>MSEDLRVGLFPVRYLVGTGLPGAPQLVLDLMVDTVDHSVVGRAAVSQAVSPPLNFHADVWGSYVFRLGPPPRRDGSGAIVQISLQGNQGGPQSNSMITFYGELLLKGDGKTGVASYRYYSNGSWHEVENVPVKADPELVPIEPGPVIGQSSMSAIGSAAMYGVAIQSAAASGDLAHMRTLSAYARQQLESRDEIAAALSELKAEIAKLESRQHHHHHH[2x]

The Q63NT7 protein from Burkholderia pseudomallei is 212 amino acids in length (molecular mass 22.5 kDa). It contains two predicted domains: an N-terminal domain of unknown function (14.5 kDa; DUF1842) and the C-terminal domain (DUF1843; 5.4 kDa), which tends to appear in multiple paralogous copies within individual bacterial operons. The N-terminal domain was predicted to fold into a β-barrel composed of eight antiparallel strands. Polar residues are found covering the exterior surface of the β-barrel, while the interior of the β-barrel is lined with mostly hydrophobic residues, without space for a channel through the barrel.

Finally, we continued to optimize the crystallization conditions and identified another condition that grew well diffracting needle-shaped crystals that were suitable for data collection on the synchrotron microfocus beamline. We were able to collect a complete data set from a single crystal, which could be processed in space group P212121. We refer to this crystal as form 3, since its unit-cell dimensions were distinct from those of forms 1 and 2. Form 1 crystals gave a combined LLG value of 719, form 2 crystals gave an LLG value of 394 and form 3 crystals gave an LLG value of 305. Importantly, the Phaser statistics for molecular-replacement solutions using the refined form 1 crystal structure were much improved over those from AlphaFold-predicted models; the form 2 data set gave a Phaser LLG value of 624, while the form 3 data set gave a Phaser LLG value of 662 (compared with LLGs of 394 and 305 for the AlphaFold models). The form 3 model had an R factor of 27.3% and an R free of 33.3%. The backbone r.m.s.d. values between the experimental structures and the AlphaFold model were 0.35 Å for form 1, 0.49 Å for form 2 and 0.46 Å for form 3. As a result, no biologically relevant interfaces could be inferred with confidence. One potentially relevant exception is that the form 2 noncrystallographic interface is present as a crystallographic interface in the form 3 crystals.>[2x]MPRQASTFTNPVLWEDHPDLEVFRVGSVFYYSSSTFAYSPGAPVLKSYDLVHWTPVTHSVPRLNFGSNYDLPSGTPGAYVKGIWASTLRYRRSNDRFYWYGCVEGRTYLWTSPGGNALANNGEVPPSAWNWQHTATIDNCYYDAGLLIDDDDTMYIAYGNPTINVAQLSPDGTRQVRVQQRVYAHPQGQTVEGARMYKIRGNYYILVTRPADAEYVLRSTTGSPFGPYEARTLVSRIQGPLANAGFA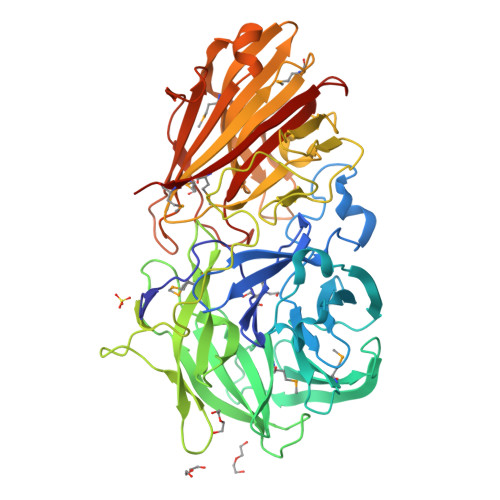HQGGIVDAPDGTWHYVAFMDAYPGGRIPVVAPLRWTADGWPEVVTDSQGRWGTSYPIPVRGAKNATEGLASTDLDEFRGTRFSEHWEWNHNPDTSKFTLLGGNEGGLILRTATVTGDLFAARNTLTRRIAGPKASGIFRLDVRGMRDGDRAGAVLFRDRAAYIGVWKQGNEARIVMVDDLRLNEDGWRTASTGRVAANGPVIDTNAQQDIWLRIDADITPAFGTNTERTTTFYYSIDGGRTYTRLGPAFAMTNSWRYFTGYRFGVFNFSTKSLGGEVKVKGFKMNMILEHHHHHH>[2x]DEQPEPRTRRRAYLWCKEFLPGAWRGLREDEFHISVIRGGLSNMLFQCSLPDTTATLGDEPRKVLLRLYGAILQMRSCNKEGSEQAQKENEFQGAEAMVLESVMFAILAERSLGPKLYGIFPQGRLEQFIPSRRLDTEELSLPDISAEIAEKMATFHGMKMPFNKEPKWLFGTMEKYLKEVLRIKFTEESRIKKLHKLLSYNL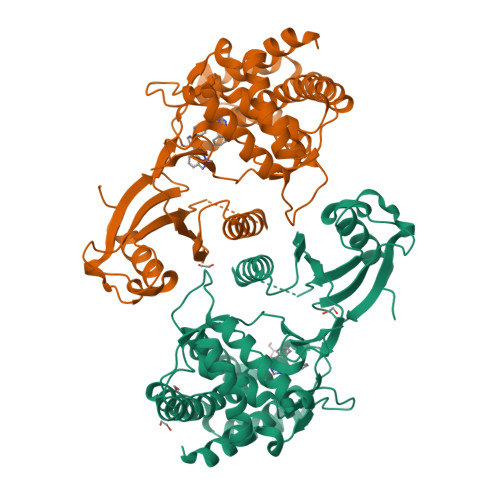PLELENLRSLLESTPSPVVFCHNDCQEGNILLLEGRENSEKQKLMLIDFEYSSYNYRGFDIGNHFCEWMYDYSYEKYPFFRANIRKYPTKKQQLHFISSYLPAFQNDFENLSTEEKSIIKEEMLLEVNRFALASHFLWGLWSIVQAKISSIEFGYMDYAQARFDAYFHQKRKLGV>[4x]MYKDLEGKVVVITGSSTGLGKSMAIRFATEKAKVVVNYRSKEDEANSVLEEIKKVGGEAIAVKGDVTVESDVINLVQSAIKEFGKLDVMINNAGLANPVSSHEM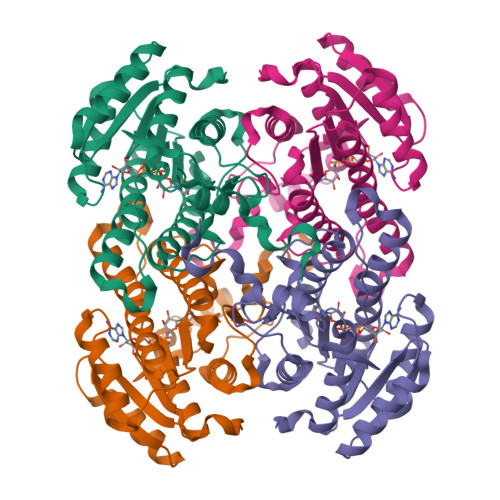SLSDWNKVIDTNLTGAFLGSREAIKYFVENDIKGTVINMSSVHEKIPWPLFVHYAASKGGMKLMTETLALEYAPKGIRVNNIGPGAINTPINAEKFADPEQRADVESMIPMGYIGEPEEIAAVAAWLASSEASYVTGITLFADGGMTQYPSFQAGRG>[4x]GSNGKLRQWLIDQIDSGKYPGLVW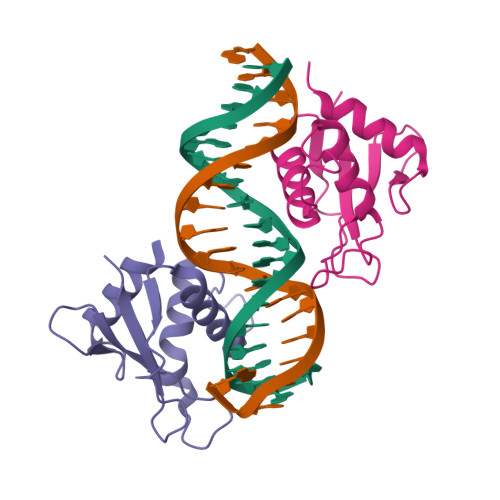ENEEKSIFRIPWKHAGKQDYNREEDAALFKAWALFKGKFREGIDKPDPPTWKTRLRCALNKSNDFEELVERSQLDISDPYKVYRIVP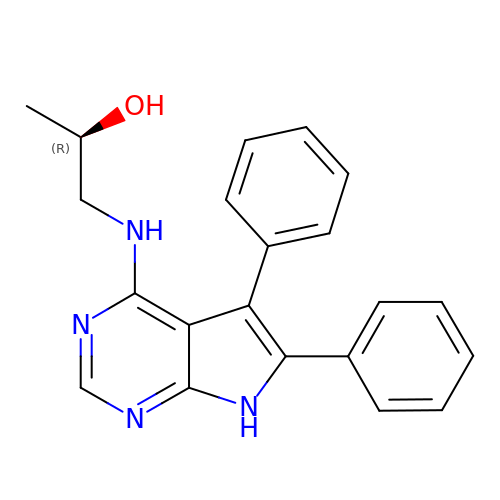(2R)-1-[(5,6-DIPHENYL-7H-PYRROLO[2,3-D]PYRIMIDIN-4-YL)AMINO]PROPAN-2-OL | C21 H20 N4 O | VBASHTSSQNDDAS-CQSZACIVSA-N>SEDNITVRFVTENDKEGWQRLWKSYQDFYEVSFPDDLDDFNFGRFLDPNIKMWAAVAVESSSEKIIGMINFFNHMTTWDFKDKIYINDLYVDENSRVKGAGGKLIQFVYDEADKLGTPSVYWCTDESN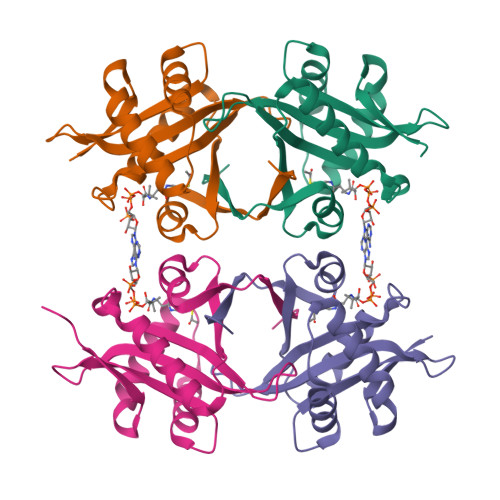HRAQLLYVKVGYKAPKILYKRKGY[4x]> MVNTEEDGLPRLIDAIEEASKIPAKRRQTPIKPTI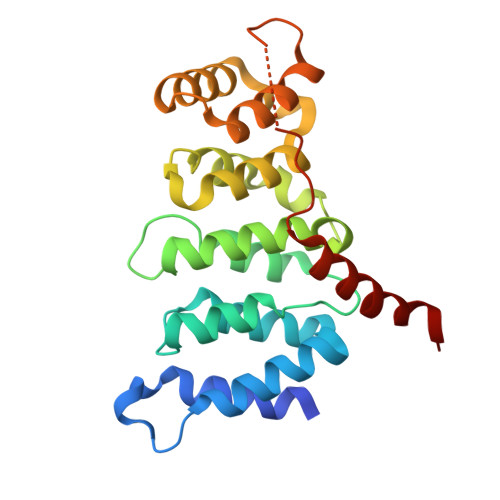EKLTTHLYTHGASPDSLLRLADLLTLRNHLDQASLAAITRNLYPSSTVSDEVVLRFIGALGHGQLKPTLALQALFLRWLVMVYHLLENPGVLGQVYGVLFDLLDTAAIRPQLCHLLALVTRRKHVRPFRIQAILTLSRQTGGDPNLTGLLRVFKNYYPEIIVGDATKGRASAFKHPDPQWRQHLDEIQQRRSEA> SNAHLKNNQTLANGATVTIYPTTTEPTNYVVYLHGGGMIYGTKSDLPEELKELFTSNGYTVLALDYLLAPNTKIDHILRTLTETFQLLNEEIIQNQSFGLCGRSAGGYLMLQLTKQLQTLNLTPQFLVNFYGYTDLEFIKEPRKLLKQAISAKEIAAIDQTKPVWDDPFLSRYLLYHYSIQQALLPHFYGLPENGDWSAYALSDETLKTFPPCFSTASSSDEEVPFRYSKKIG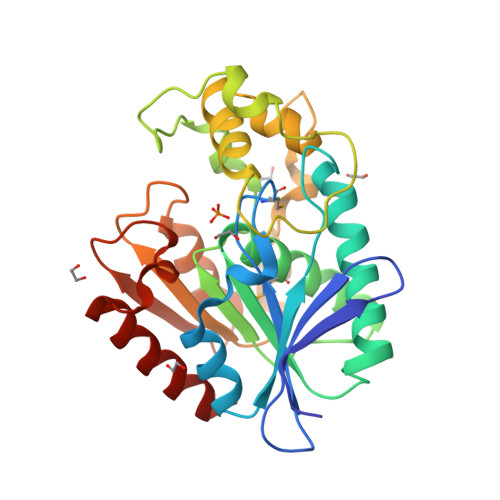RTIPESTFKAVYYLEHDFLKQTKDPSVITLFEQLDSWLKER> GSHMGSNQKRGVKVLKQELGGLGISIKGGKENKMPILISKIFKGLAADQTQALYVGDAILSVNGADLRDATHDEAVQALKRAGKEVLLEVKYMREGSAYGSVKAYTNFDAERDALNIETAIKTKGVDEVTIVNILT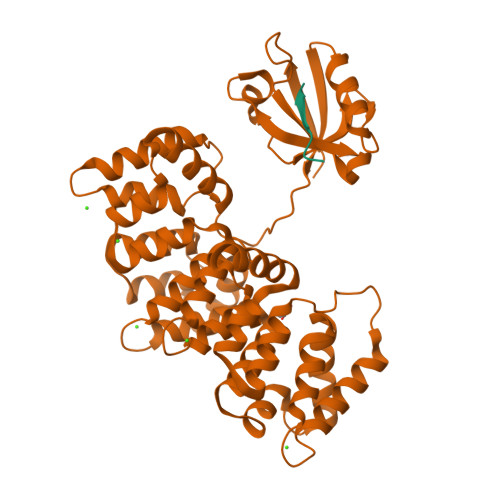NRSNEQRQDIAFAYQRRTKKELASALKSALSGHLETVILGLLKTPAQYDASELKASMKGLGTDEDSLIEIICSRTNQELQEINRVYKEMYKTDLEKDIISDTSGDFRKLMVALAKGRRAEDGSVIDYELIDQDARDLYDAGVKRKGTDVPKWISIMTERSVPHLQKVFDRYKSYSPYDMLESIRKEVKGDLENAFLNLVQCIQNKPLYFADRLYDSMKGKGTRDKVLIRIMVSRSEVDMLKIRSEFKRKYGKSLYYYIQQDTKGDYQKALLYLCGGDD;> TDDSKPTRRETEV>[2x]SQEADKMFFLIEKIKMFNQDIEKLVEGEEVVRENETRLYNKIREDFKNWVGILATNTQKVKNIIHEEVEKYEKQAAAAELLGFVNYKTFEIIVHQYIQQLVE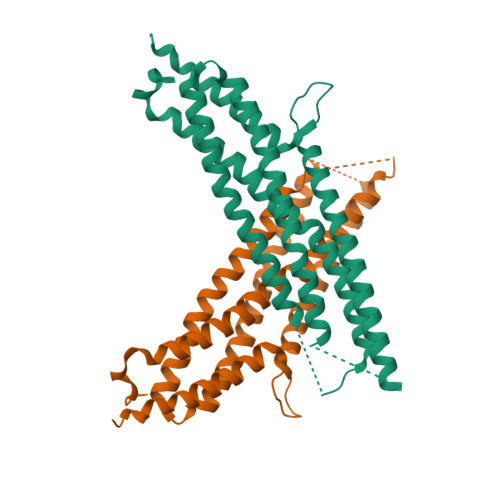PALSMLQKAMEIIQQAFINVAKKHFGEFFNLNQTVQSTIEDIKVKHTAKAENMIQLQFRMEQMVFKLNSHFPSNESSVSSFTEIGIHLNAYFLETSKRLANQIPFIIQYFMLRENGDSLQKAMMQILQEKNRYSWLL> MAPKSSSSGSKKKSSASSNSADAKASKFKLPAEFITRPHPSKDHGKETCTAYIHPNVLSSLEINPGSFCTVGKIGENGILVIARAGDEEVHPVNVITLSTTIRSVGNLILGDRLELKKAQVQPPYATKVTVGSLQGYNILECMEEKVIQKLLDDSGVIMPGMIFQNLKTKAGDESIDVVITDASDDSLPDVSQLDLNMDDMYGGLDNLFYLSPPFIFRKGSTHITFSKETQANRKYNLPEPLSYAAVGGLDKEIESLKSAIEIPLHQPTLFSSFGVSPPRGILLHGPPGTGKTMLLRVVANTSNAHVLTINGPSIVSKYLGETEAALRDIFNEARKYQPSIIFIDQIDSIAPNRANDDSGEVESRVVATLLTLMDGMGAAGKVVVIAATNRPNSVDPALRRPGRFDQEVEIGIPDVDARFDILTKQFSRMSSDRHVLDSEAIKYIASKTHGYVGADLTALCRESVMKTIQRGLGTDANIDKFSLKVTLKDVESAMVDIRPSAMREIFLEMPKVYWSDIGGQEELKTKMKEMIQLPL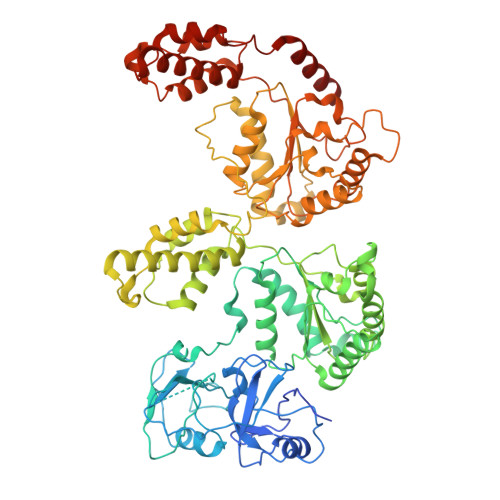EASETFARLGISAPKGVLLYGPPGCSKTLTAKALATESGINFLAVKGPEIFNKYVGESERAIREIFRKARSAAPSIIFFDQIDALSPDRDGSSTSAANHVLTSLLNEIDGVEELKGVVIVAATNRPDEIDAALLRPGRLDRHIYVGPPDVNARLEILKKCTKKFNTEESGVDLHELADRTEGYSGAEVVLLCQEAGLAAIMEDLDVAKVELRHFEKAFKGIARGITPEMLSYYEEFALRSGSSS> SNAQADIALIGLAVMGQNLILNMNDHGFVVCAFNRTVSKVDDFLANEAKGTKVVGAQSLKEMVSKLKKPRRIILLVKAGQAVDDFIEKLVPLLDTGDIIIDGGNSEYRDTTRRCRDLKAKGILFVGSGVSGGEEGARYGPSLMPGGNKEAWPHIKTIFQGIAAKVGTGEPCCDWVGDEGAGHFVKMVHNGIEYGDMQLICEAYHLMKDVLGMAQDEMAQAFEDWNKTELDSFLIEITANILKFQDTDGKHLLPKIRDSAGQKGTGKWTAISALEYGVPVTLIGEAVFARCLSSLKDERIQASKKLKGPQKFQFDGDKKSFLEDIRKALYASKIISYAQGFMLLRQAATEFGWTLNYGGIALMWRGGCIIRSVFLGKIKDAFDRNPELQNLLLDDFFKSAVENCQDSWRRAVSTGVQAGI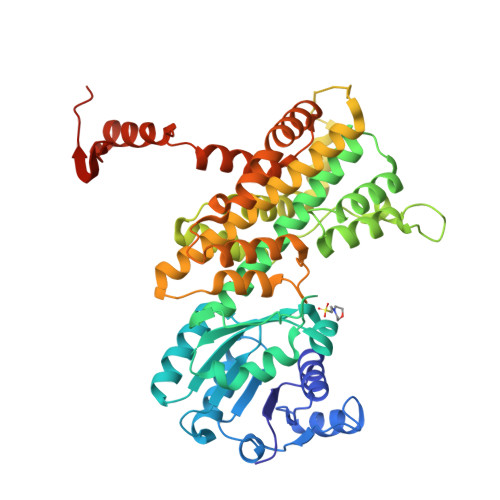PMPCFTTALSFYDGYRHEMLPASLIQAQRDYFGAHTYELLAKPGQFIHTNWTGHGGTVSSSSYNA>[4x]ASKWTYFGPDGENSWSKKYPSCGGLLQSPIDLHSDILQYDASLTPLEFQGYNLSANKQFLLTNNGHSVKLNLPSDMHIQGLQSRYSATQLHLHWGNPNDPHGSEHTVSGQHFAAELHIVHYNSDLYPDASTASNKSEGLAVLAVLIEMGSFNPSYDKIFSHLQHVKYKGQEAFVPGFNIEELLPERTAEYYRYRGSLTTPPCNPTVLWTVFRNPVQISQEQLLALETA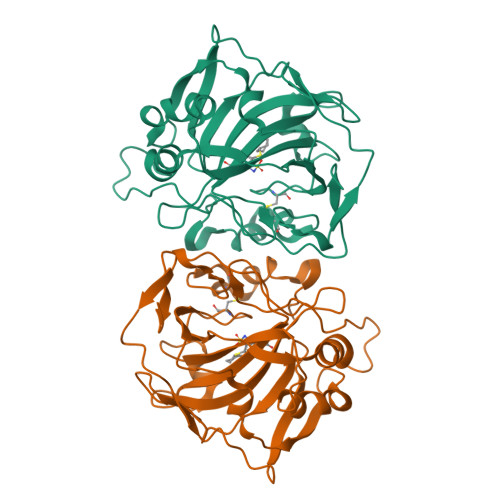LYCTHMDDPSPREMINNFRQVQKFDERLVYTSFSQ> GIQGLAKLIADVAPSAIRENDIKSYFGRKVAIDASMSIYQFLIAVRQGGDVLQNEEGETTSHLMGMFYRTIRMMENGIKPVYVFNGKPPQLKSGELAKRSERRAEAEKQLQQAQAAGAEQEVEKFTKRLVKVTKQHNDECKHLLSLMGIPYLDAPSEAEASCAALVKAGKVYAAATEDMDCLTFGSPVLMRHLTASEAKKLPIQEFHLSRILQELGLNQEQFVDLCILLGSDYCESIRGIGPKRAVDLIQKHKSIEEIVRRLDPNKYPVPENWLHKEAHQLFLEPEVLDPESVELKWSEPNEEELIKFMCGEKQFSEERIRSGVKRLSKSRQGSTLEVLFQ

The structure-specific nuclease, flap endonuclease-1 (FEN1) plays a vital role in maintaining genome integrity by precisely processing intermediates of Okazaki fragment maturation, long-patch excision repair, telomere maintenance, and stalled replication forks. FEN1 preferentially binds to double flap substrates with a one nt 3′-flap and any length of 5′-flap, including zero. It catalyses a single hydrolytic incision one nucleotide (nt) into dsDNA to yield nicked DNA ready for direct ligation. Here crystallographic analyses uncover an unprecedented electrostatic steering of an inverted 5′-flap through the human FEN1 (hFEN1) helical gateway.

In the hFEN1-D86N and hFEN1-R100A structures, the ssDNA (5′-flap) region of the substrate threaded through the tunnel formed by the gateway/cap. In the hFEN1-D86N structure, two basic residues of the gateway/cap, Arg104 and Lys132, were within 4–7 Å of the +1, +2 and +3 phosphodiester. In the hFEN1-D86N structure, we were surprised that the scissile phosphate was within catalytic distance of the active site while surrounding bases remained basepaired to the template strand. In striking contrast, the scissile phosphodiester bond was directly coordinated to the one active site metal ion in the hFEN1-D86N structure. Furthermore, the +1 and −1 nts remained unexpectedly basepaired to the template strand, which is shifted relative to the other substrate structures via a dsDNA distortion surrounding the scissile phosphodiester. There is no base stacking between −1 and −2 nts in the 5′-flap strand; instead, an unusual interstrand base stacking interaction occurs between the −2 nt of the 5′-flap strand and the template strand opposite of the −1 nt. In concert with the DNA rotation in hFEN1-D86N, Tyr40 is in a different rotamer conformation from all other substrate or product bound or DNA-free hFEN1 structures. The Tyr ring is fully stacked on the +1 base, and its side chain hydroxyl forms a hydrogen bond to the +1 phosphate. In the hFEN1-D86N-substrate structure, cap and gateway helices 4 and 5 are shifted 1–3 Å towards the dsDNA relative to all other hFEN1 crystal structures with DNA. Close examination of the hFEN1-D86N structure revealed a water molecule 3.3 Å from the scissile phosphate.>MGSSHHHHHHSQDPGFEFTLMVVGESGLGKSTLINSLFLTDLYSPEYPGPSHRIKKTVQVEQSKVLIKEGGVQLLLTIVDTPGFGDAVDNSNCWQPVIDYIDSKFEDYLNAESR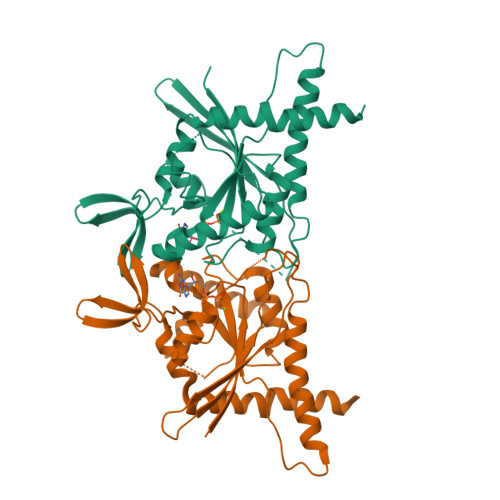VNRRQMPDNRVQCCLYFIAPSGHGLKPLDIEFMKRLHEKVNIIPLIAKADTLTPEECQQFKKQIMKEIQEHKIKIYEFPETDDEEENKLVKKIKDRLPLAVVGSNTIIEVNGKRVRGRQYPWGVAEVENGEHCDFTILRNMLIRTHMQDLKDVTNNVHYENYRSRKLAAVT[2x]> RRRKPRVLFSQAQVYELERRFKQQRYLSAPERDQLASVLKLTSTQVKIW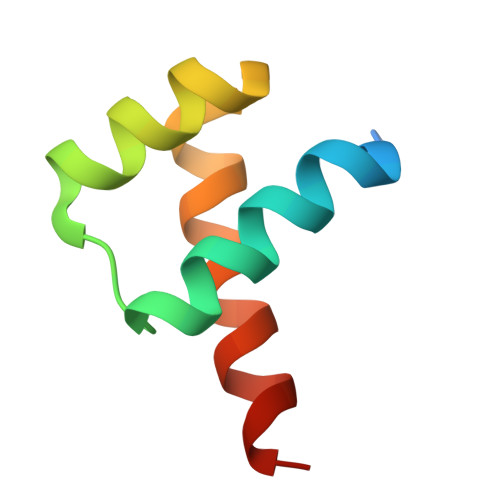FQNRRYKSKRQR>[4x]MSLGRFVRHALITAGT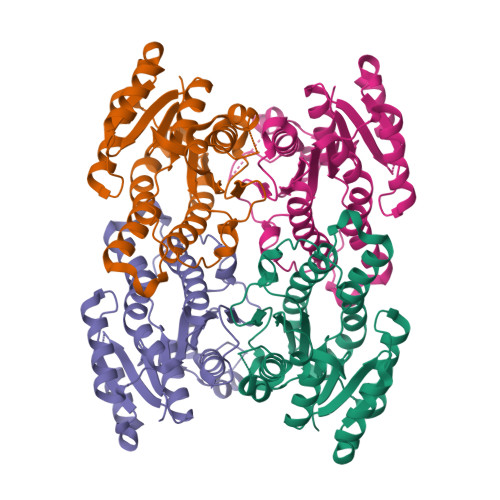KGLGKQVTEKLLAKGYSVTVTYHSDTTAMETMKETYKDVEERLQFVQADVTKKEDLHKIVEEAMSHFGKIDFLINNAGPYVFERKKLVDYEEDEWNEMIQGNLTAVFHLLKLVVPVMRKQNFGRIINYGFQGADSAPGWIYRSAFAAAKVGLVSLTKTVAYEEAEYGITANMVCPGDIIGEMKEATIQEARQLKEHNTPIGRSGTGEDIARTISFLCEDDSDMITGTIIEVTGAVDVIHREGHHHHHH>[2x]QGNDTSEVMLLDTGWEFSQSGTEKWMPATVPGTVHQDLISHELLPNPFYGMNEKKIQWVENEDWEYRTSFIVSEEQLNRDGIQLIFEGLDTYADVYLNGSLLLKADNMFVGYTLPVKSVLRKGENHLYIYFHSPIRQTLPQYASNGFNYPADNDHHEKHLSVFSRKAPYSYGWDWGIRMVTSGVWRPVTLRFYDIATISDYYVRQLSLTDENARLSNELIVNQIVPQKIPAEVRVNVSLNGTTVTEVKQQVTLQPGINHITLPAEVTNPVRWMPNGWGTPTLYDFSAQIACGDRIVAEQSHRIGLRTIRVVNEKDKDGESFYFEVNGIPMFAKGANYIPQDALLPNVTTERYQTLFRDMKEANMNMVRIWGGGTYENNLFYDLADENGILV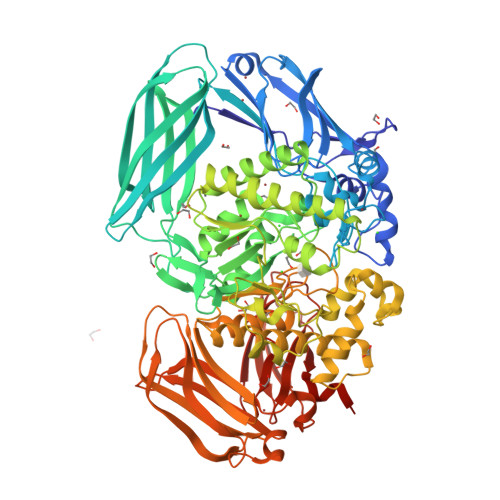WQDFMFACTPYPSDPTFLKRVEAEAVYNIRRLRNHASLAMWCGNNEILEALKYWGFEKKFTPEVYQGLMHGYDKLFRELLPSTVKEFDSDRFYVHSSPYLANWGRPESWGTGDSHNWGVWYGKKPFESLDTDLPRFMSQFGFQSFPEMKTIAAFAAPEDYQIESEVMNAHQKSSIGNSLIRTYMERDYIIPESFEDFVYVGLVLQGQGMRHGLEAHRRNRPYCMGTLYWQLNDSWPVVSWSSIDYYGNWKALHYQAKRAFAPVLINPIQQNDSLSVYLISDRLDTMEQMTLEMKVVDFDGKTLGKKIQVHSLEVPANTSKCVYRAKLDGWLTPEDCRRSFLKLILKDKSGHQVAESVHFFRKTKDLQLPPTSVSYQMKQTDGKCELTLFSSMLAKDIFIETPLQGARYSDNFFDLLPGERKKVIITSPRIKKGEELPVNIKHIRETYKLEHHHHHH> VFHKIRNEDLIFNESLGQGTFTKIFKGVRREVGDYGQLHETEVLLKVLDKAHRNYSESFFEAASMMSKLSHKHLVLNYGVCFCGDENILVQEFVKFGSLDTYLKKNKNCINILWKLEVAKQLAWAMHFLEENTLIHGNVCAKNILLIREEDRKTGNPPFIKLSDPGISIT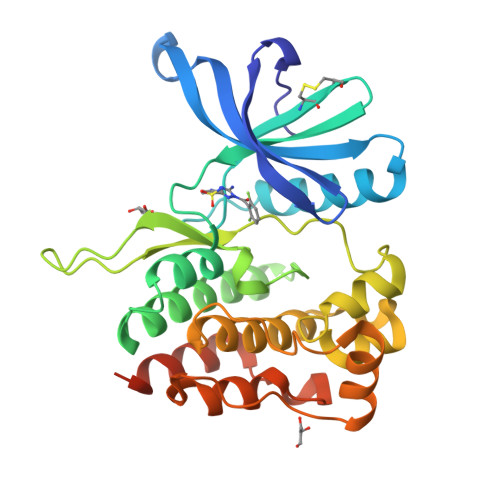VLPKDILQERIPWVPPECIENPKNLNLATDKWSFGTTLWEICSGGDKPLSALDSQRKLQFYEDRHQLPAPKAAELANLINNCMDYEPDHRPSFRAIIRDLNSLFTPDLVPRGSHHHHHH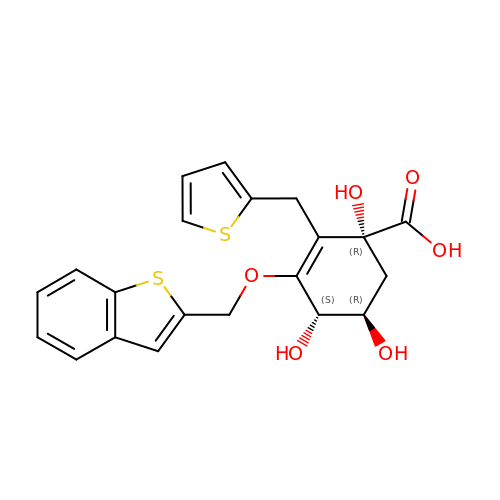(1R,4S,5R)-3-(BENZO[B]THIOPHEN-2-YL)METHOXY-1,4,5-TRIHYDROXY-2-(THIEN-2-YL)METHYLCYCLOHEX-2-EN-1-CARBOXYLATE | C21 H20 O6 S2 | ILDPLWRWUROBLZ-PLMTUMEDSA-N> GD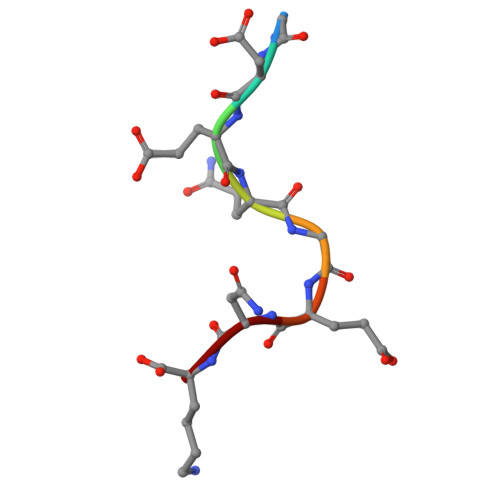EQGENK>MHHHHHHMANCERTFIAIKPDGVQRGLVGEIIK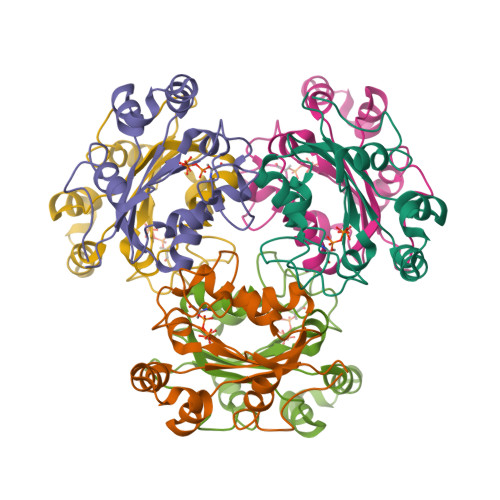RFEQKGFRLVGLKFMQASEDLLKEHYVDLKDRPFFAGLVKYMHSGPVVAMVWEGLNVVKTGRVMLGESNPADSKPGTIRGDFCIQVGRNIIHGSDSVESAEKEIGLWFHPEELVDYT[6x]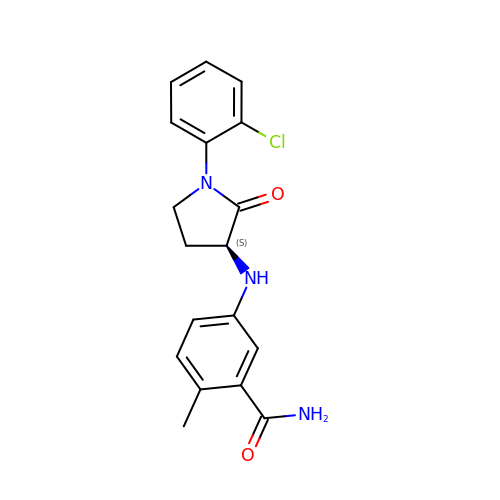5-[[(3S)-1-(2-chlorophenyl)-2-oxidanylidene-pyrrolidin-3-yl]amino]-2-methyl-benzamide | C18 H18 Cl N3 O2 | QGUKHHBQJVYLMV-HNNXBMFYSA-N>MGSDKIHHHHHHLKMKKYTKTHEWVSIEDKVATVGITNHAQEQLGDVVYVDLPEVGREVKKGEVVASIESVK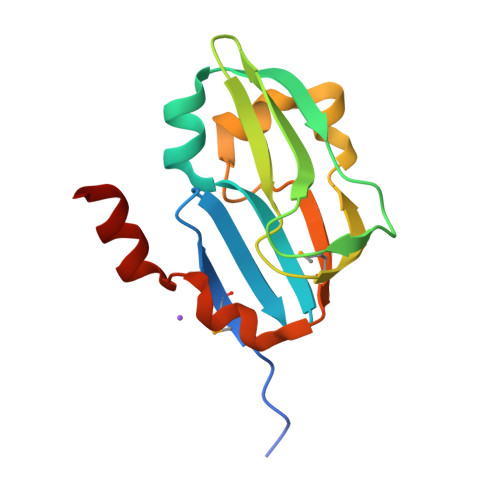AAADVYAPLSGKIVEVNEKLDTEPELINKDPEGEGWLFKMEISDEGELEDLLDEQAYQEFCAQE[2x]> GAMEPSAPKELKFGDITKDSVHLTWEPPDDDGGSPLTGYVVEKREVSRKTWTKVMDFVTDLEFTVPDLVQGKEYLFKVCARNKCGPGEPAYVDEPVNMS

Titin is a giant, elastic, sarcomeric protein with a molecular weight of more than 3800 kD. Titin consists primarily of two types of protein domains: fibronectin type III (FnIII) domains and immunoglobulin (Ig) domains (ca 100 residues in length) that account for over 90% of its mass. Despite the repetitive composition of titin, a single main immunogenic region (MIR) has so far been identified in its chain that elicits the reactivity of almost all known anti-titin antibodies in MG patients. This 30 kD segment, also termed MGT30, consists of a domain triplet of composition Ig-FnIII-FnIII located in the titin segment at the junction of the I- and A-bands (I/A) and corresponding to domains 4 to 6 in this region of the chain, i.e., tandem I109-I111 also termed I/A4-I/A6, (nomenclature as in Bang et al., 2001).

To gain an insight into the possible molecular determinants of I110 recognition by anti-titin antibodies, we elucidated the 3D-structure of the isolated I110 domain, the double tandem I110-I111 and the full-length MIR region I109-I110 using X-ray crystallography. Domain I110 also presented such typical features without detectable deviations. In fact, its structural comparison to FnIII domains from titin with known 3D-structure revealed a remarkable agreement: namely, RMSDCα values for superimpositions onto domains A77, A78 and A170 yielded values of 0.81 Å, 1.02 Å and 1.18 Å, respectively. The I110 domain showed a stable and same structure when isolated and arrayed with its neighboring domains. In the present study, we clearly showed that the single antigenic region of the titin MIR is its middle FnIII domain, I110. In another two Western blots, four more anti-titin sera and two HC were also tested with the same result. These results suggested that the antibody epitope in I110 is formed by a linear sequence motif and is not the result of a three-dimensional, spatial arrangement of amino acid residues with specific conformation. In brief, structural analysis did not lead to the identification of unique features in I110 that might support its unique recognition by anti-titin antibodies. An analysis of sequence conservation relative to FnIII used as negative controls in this study reveals a subset of surface residues unique to I110, that could mediate its specific recognition by anti-titin antibodies. The available crystal structures will support future studies that could resolve the role of these candidate residues in I110′s antigenicity and permit mapping their formation of epitope(s).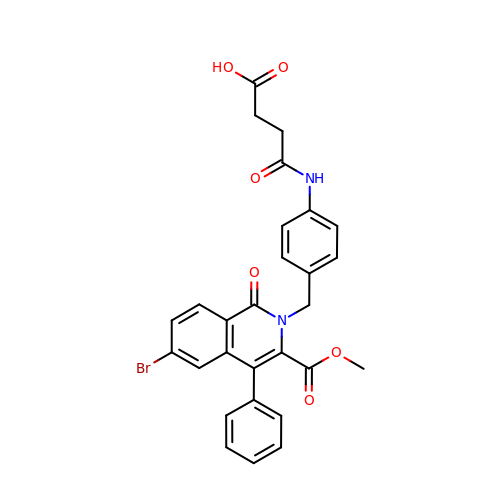4-[(4-{[6-bromo-3-(methoxycarbonyl)-1-oxo-4-phenylisoquinolin-2(1H)-yl]methyl}phenyl)amino]-4-oxobutanoic acid | C28 H23 Br N2 O6 | UJOQZQKRUNERFC-UHFFFAOYSA-N>PIIDQGPLPTLTDGDKKAINKIWPKIYKEYEQYSLNILLRFLKCFPQAQASFPKFSTKKSNLEQDPEVKHQAVVIFNKVNEIINSMDNQEEIIKSLKDLSQKHKTVFKVDSIWFKELSSIFVSTI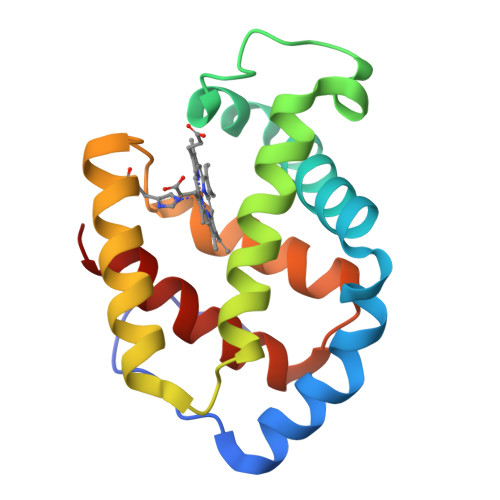DGGAEFEKLFSIICILLRSAY[2x]>NECRIERLNALEPTRTVRSEAGVTDYFDEDNEQFRCAGVSTIRRVIEPRGLLLPSMSNAPRLVYIVQGRGIVGLVMPGCPETFQSFQRSEREEGERHRWSRDEHQKVYQFQEGDVLAVPNGFAYWCYNNGENPVVAITVLDTSNDANQLDRSHRQFLLAGRQEQGRQRYGREGSIKENILRGFSTELLAAAFG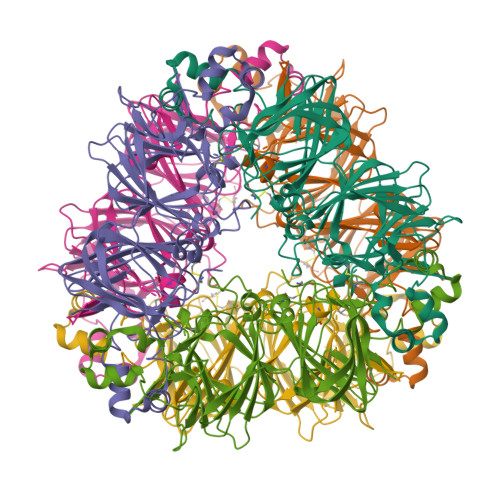VNMELARKLQCRDDTRGEIVRAENGLQVLRPSGMEEEEREEGRSINGFEETYCSMKIKQNIGDPRRADVFNPRGGRITTLNSEKLPILRFIQMSAERVVLYRNAMVSPHWNINAHSIMYCTGGRGRVEVADDRGETVFDGELRQGQLLIVPQNFAMLERAGSEGFQLVSIKTSDRAMVSTIVGKTSALRGMPVEVLMNSYRLSRDEARRVKLTRGDEVAIFTPRRESRAEA[2x]> VETISFSFSEFEPGNDNLTLQGAALITQSGVLQLTKINQNGMPAWDSTGRTLYTKPVHMWDSTTGTVASFETRFSFSIEQPYTRPLPADGLVFFMGPTKSKPAQGYGYLGVFNNSKQDNSYQTLAVEFDTFSNPWDPPQVPHIGIDVNSIRSIKTQPFQLDNGQVANVVIKYDAPSKILHVVLVYPSSGAIYTIAEI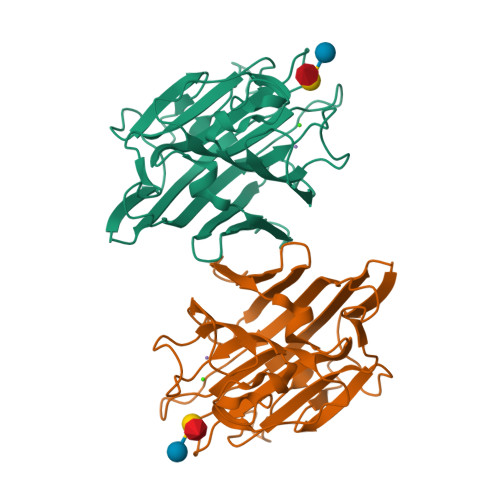VDVKQVLPDWVDVGLSGATGAQRDAAETHDVYSWSFQASLPE>[4x]QKTQSAPGTLSPVARNEKQPFYGEHQAGILTPQQAAMMLVAFDVLASDKADLERLFRLLTQRFAFLTQGGAAPETPNPRLPPLDSGILGGYIAPDNLTITLSVGHSLFDERFGLAPQMPKKLQKMTRFPNDSLDAALCHGDVLLQICANTQDTVIHALRDIIKHTPDLLSVRWKREGFISDHAARSKGKETPINLLGFKDGTANPD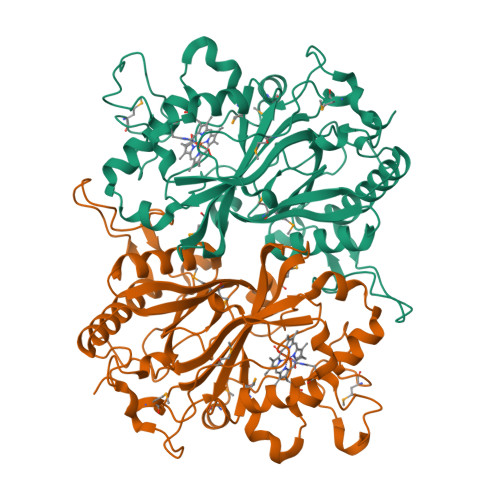SQNDKLMQKVVWVTADQQEPAWTIGGSYQAVRLIQFRVEFWDRTPLKEQQTIFGRDKQTGAPLGMQHEHDVPDYASDPEGKGIALDSHIRLANPRTAESESSLMLRRGYSYSLGVTNSGQLDMGLLFVCYQHDLEKGFLTVQKRLNGEALEEYVKPIGGGYFFALPGVKDANDYLGSALLRVLEHHHHHH>ALVFFAEDCGSNKCAIIGLM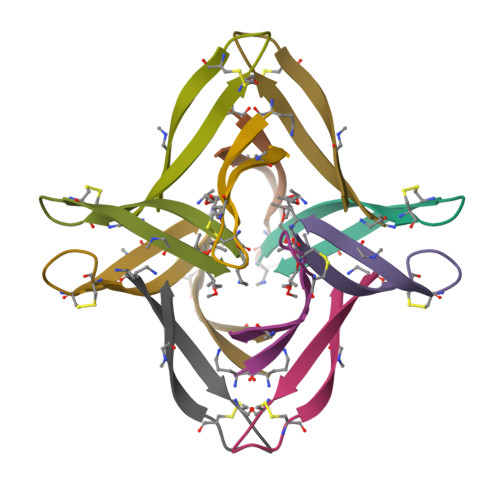V[6x]>SIVTKSIVNADAEARYLSPGELDRIKSFVSGGAQRLRIAQVLTDNRERIVKQAGDQLFQKRPDVVSPGGNAYGQEMTATCLRDLDYYLRLVTYGIVAGDVTPIEEIGIVGVREMYKSLGTPIDAVAGGVAAMKSVAAGLLSAEDAGEAGAYFDYVVGAMQ[3x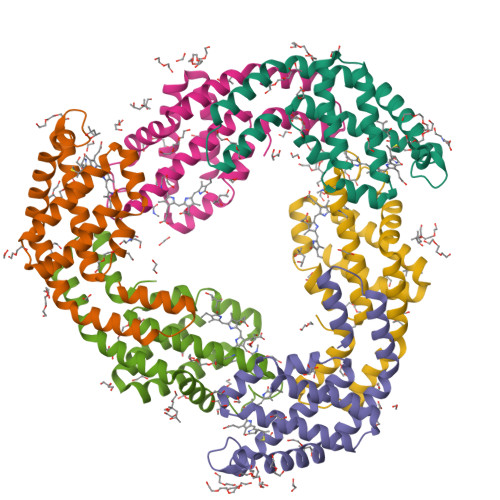];>MQDAITSVINSSDVQGKYLDNAALEKLKGYFATGELRVRAATTISANAAAIVKEAVAKSLLYSDITRPGGNMYTTRRYAACIRDLDYYLRYATYAMLAGDPSILDERVLNGLKETYNSLGVPVGATVQAIQAIKEVTASLVGPDAGKEMGVYFDYICSGLS[3x]> VPDPRGIIINLDEGELCLNSAQCKSNCCQHDTILSLLRCALKARENSE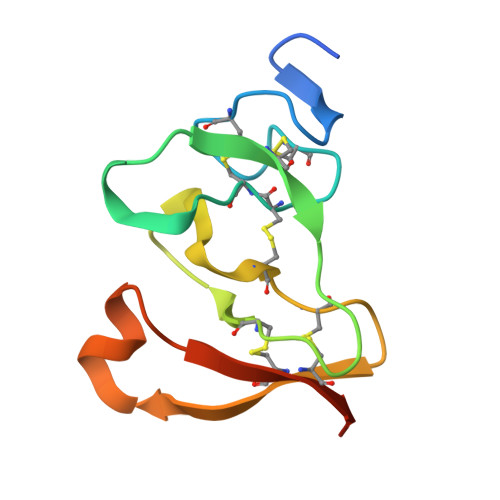CSAFTLYGVYYKCPCERGLTCEGDKSLVGSITNTNFGICHNVGRSDS> SSLDNIEMAYARQIYIYNEKIVNGHLQPNLVDLCASVAELDDKSISDMWTMVKQMTDVLLTPATDALKNRSSVEVRMEFVRQALAYLEQSYKNYTLVTVFGNLHQAQLGGVPGTYQLVRSFLNIKLPAPLPGLQDGEVEGHPVWALIYYCMRCGDLLAASQVVNRAQHQLGEFKTWFQEYMNSKDRRLSPATENKL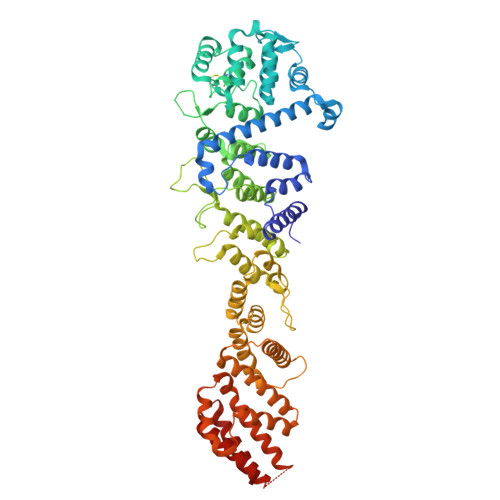RLHYRRALRNNTDPYKRAVYCIIGRCDVTDNQSEVADKTEDYLWLKLNQVCFDDDGTSSPQDRLTLSQFQKQLLEDYGESHFTVNQQPFLYFQVLFLTAQFEAAVAFLFRMERLRCHAVHVALVLFELKLLLKSSGQSAQLLSHEPGDPPCLRRLNFVRLLMLYTRKFESTDPREALQYFYFLRDEKDSQGENMFLRCVSELVIESREFDMILGKLENDGSRKPGVIDKFTSDTKPIINKVASVAENKGLFEEAAKLYDLAKNADKVLELMNKLLSPVVPQISAPQSNKERLKNMALSIAERYRAQGISANKFVDSTFYLLLDLITFFDEYHSGHIDRAFDIIERLKLVPLNQESVEERVAAFRNFSDEIRHNLSEVLLATMNILFTQFKRLKGTSPSSSSRPQRVIEDRDSQLRSQARTLITFAGMIPYRTSGDTNARLVQMEVLMN>SNAMKLMDVHVLFSGGKDSSLSAVILKKLGYNPHLITINFGVIPSYKLAEETAKILGFKHKV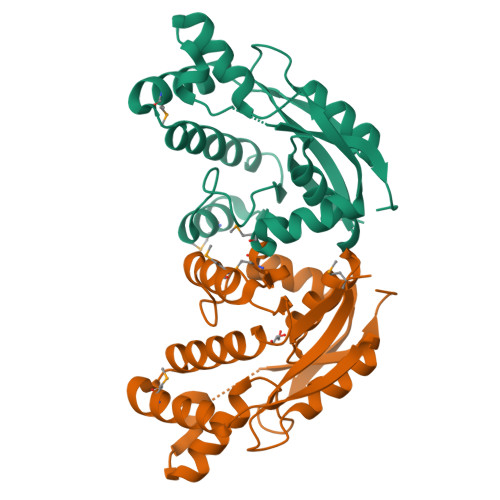ITLDRKIVEKAADMIIEHKYPGPAIQYVHKTVLEILADEYSILADGTRRDDRVPKLSYSEIQSLEMRKNIQYITPLMGFGYKTLRHLASEFFILEEIKSGTKLSSDYEAEIRHILKERGESPEKYFPEHKQTRVVGLKKEI[6x]> MKKYTCTVCAYIYNPEDGDPDNGVNPGTDFKDIPDDWVCPLC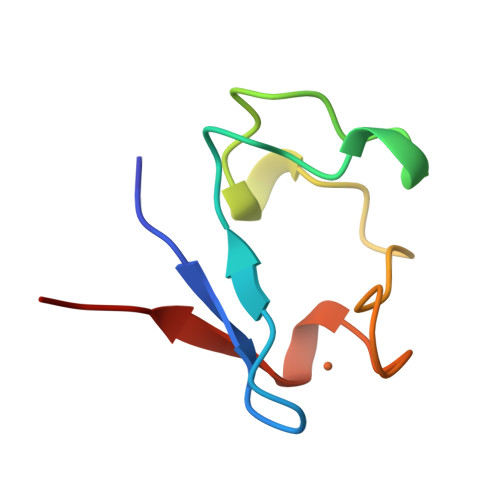GVGKDQFEEVEE> MHHHHHHMVDEILKLKKEKGYIILAHNFQIPELQDIADFVGDSLQLARKAMELSEKKILFLGVDFMAELVKILNPDKKVIVPDRSATCPMANRLTPEIIREYREKFPDAPVVLYVNSTSECKTLADVICTSANAVEVVKKLDSSVVIFGPDRNLGEYVAEKTGKKVITIPENGHCP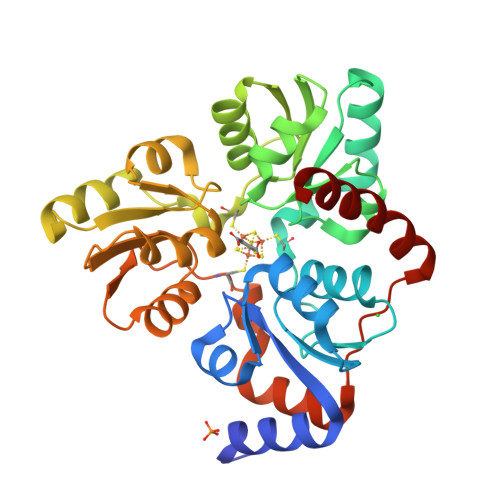VHQFNAESIDAVRKKYPDAKVIVHPECPKPVRDKADYVGSTGQMEKIPERDPSRIFVIGTEIGMIHKLKKKFPDREFVPLEMAVCVNMKKNTLENTLHALQTESFEVILPKEVIEKAKKPILRMFELMG>GSHMESFLLSKVSFVIKKIRLEKGMTQEDLAYKSNLDRTFISGIERNSRNLTIKSLELIMKGLEVSDVVFFEMLIKEILKHD[4x]

The most widespread of these mechanisms employs a “controller” (C) protein encoded by a gene downstream of its own promoter, and usually co-transcribed with the endonuclease (R) gene as a single transcriptional unit. The C-protein binds at various sites within the C/R promoter to regulate transcription of its own gene and the associated endonuclease gene. Unusually, in the RM system Esp1396I, the C-protein also represses the MTase (M) gene by binding to the promoter at the transcriptional start site, denoted OM where the C/R genes and the M gene are transcribed convergently from different promoters. Flexibility in this loop is very important for DNA sequence recognition, as it has been observed in the nucleoprotein structures to adopt different conformations depending on which operator site the protein is bound to.

We also crystallized one of the mutant proteins bound to DNA and have determined the structure of this DNA-protein complex, to compare the conformation of the DNA in the native and mutant complexes. The DNA duplex was designed with overhanging A-T bases that, in the crystal, formed a pseudo-continuous DNA double helix. The overall Y37F-19OM structure was essentially identical to the native complex, with an RMSD of 0.5 Å for the main chain protein atoms. The three major DNA base-binding residues R35, T36 and R46 were in essentially the same positions as those observed in the WT-19OM co-crystal structure, making the same interactions. The structure of the DNA duplex in the Y37F-19OM co-crystal structure also closely resembles that in the native complex, with an overall RMSD of 0.6 Å. The tyrosine residue Y37 in C.Esp1396I is implicated in DNA bending due to its interaction with the phosphate group at the highly compressed minor groove in all the known C-protein-DNA structures. However, we find that the overall bend angles of the DNA in the Y37F-19OM and WT-19OM complexes are effectively identical at 54.7° and 56.0°, respectively. This would suggest that the missing hydroxyl from the tyrosine, and concomitant loss of a key hydrogen bond interaction, does not affect the DNA distortion induced by C.Esp1396I. Comparing the native and mutant (Y37F) protein-DNA complex structures, the tyrosine and the phenylalanine were equally buried and inaccessible to solvent and in both cases the phenyl ring stacks against the deoxyribose ring in the DNA. From the Y37F-19OM co-crystal structure, it is clear that the only major alteration to the binding interface is the loss of the hydroxyl - phosphate hydrogen bonds, of which there is one per protein subunit.>[2x]AMAISDPQSSTRNELETG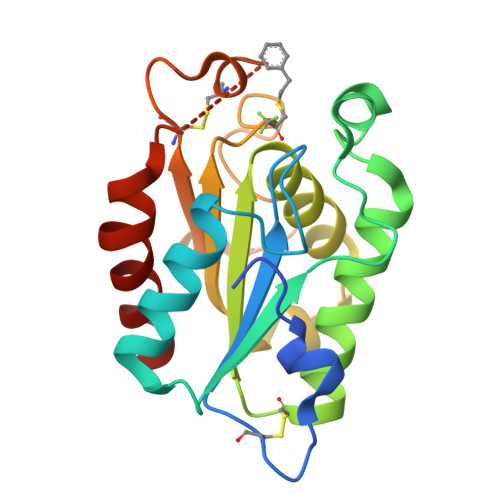SSSACPKVIYIFARASTEPGNMGISAGPIVADALERIYGANDVWVQGVGGPYLADLASNFLPDGTSSAAINEARRLFTLANTKCPNAAIVSGGYSQGTAVMAGSISGLSTTIKNQIKGVVLFGYTKNLQNLGRIPNFETSKTEVYCDIADAVCYGTLFILPAHFLYQTDAAVAAPRFLQARIG>[4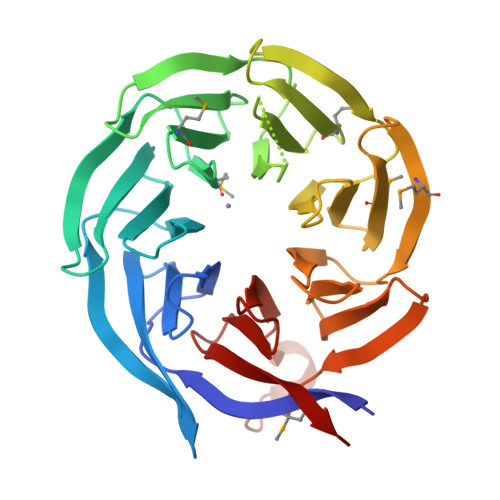x]MASNEVLVLRGTLEGHNGWVTSLATSAGQPNLLLSASRDKTLISWKLTGDDQKFGVPVRSFKGHSHIVQDCTLTADGAYALSASWDKTLRLWDVATGETYQRFVGHKSDVMSVDIDKKASMIISGSRDKTIKVWTIKGQCLATLLGHNDWVSQVRVVPNEKADDDSVTIISAGNDKMVKAWNLNQFQIEADFIGHNSNINTLTASPDGTLIASAGKDGEIMLWNLAAKKAMYTLSAQDEVFSLAFSPNRYWLAAATATGIKVFSLDPQYLVDDLRPEFAGYSKAAEPHAVSLAWSADGQTLFAGYTDNVIRVWQVMTAN> MEHVAFGSEDIENT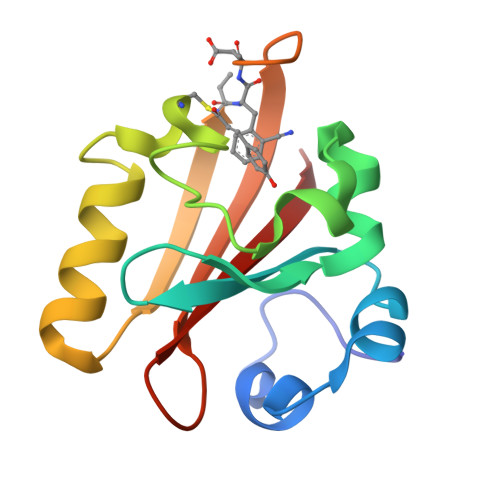LAKMDDGQLDGLAFGAIQLDGDGNILQYNAAEGDITGRDPKQVIGKNFFKDVAPCTDSPEFYGKFKEGVASGNLNTMFEYTXDYQKTPTKVKVHMKKALSGDSYWVFVKRV>[4x]RNDCVLDVMHAIYQQNKEHFQDECTKLLVGNIVITRYNNRTYRIDDVDWNKTPKDSFTMSDGKEITFLEYYSKNYGITVKEEDQPLLIHRPSERQDNHGMLLKGEILL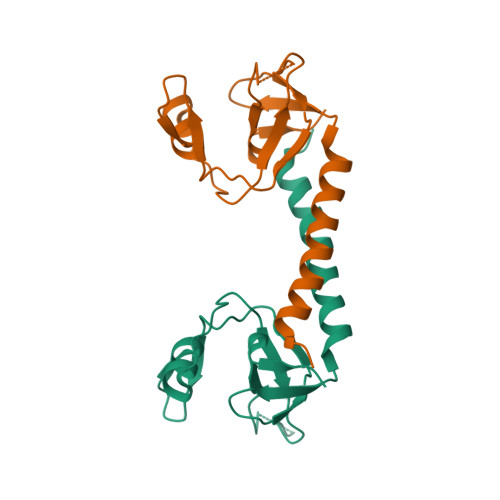LPELSFMTGIPEKMKKDFRAMKDLAQQINLSPKQHHSALE9-(5,5-DIFLUORO-5-PHOSPHONOPENTYL)GUANINE | C10 H14 F2 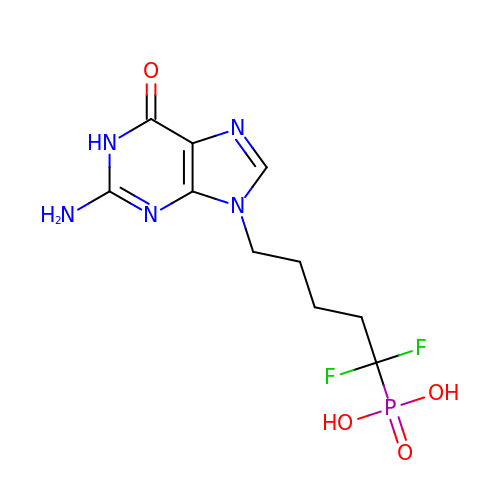N5 O4 P | JANQQPWTLXUSCD-UHFFFAOYSA-N> FSLGLQDFDLLRVIGRGSYAKVLLVRLKKTDRIYAMKVVKKELVNDDEDIDWVQTEKHVFEQASNHPFLVGLHSCFQTESRLFFVIEYVNGGDLMFHMQRQRKLPEEHARFYSAEISLALNYLHERGIIYRDLKLDNVLLDSEGHIKLTDYGMCKEGLRPGDTTSTFCGTPNYIAPEILRGEDYGFSVDWWALGVLMFEMMAGRSPFDIVGSSDNPDQNTEDYLFQVILEKQIRIPRSLSVKAASVLKSFLNKDPKERLGCHPQTGFADIQGHPFFRNVDWDMMEQKQVVPPFKPNISGEFGLDNFDSQFTNEPVQLTPDDDDIVRKIDQSEFEGFEYINPLLMSAEECV

Atypical protein kinase C (aPKC) is a key apical-basal polarity determinant and Par complex component. The atypical protein kinase C (aPKC in Drosophila or PKCι/PKCζ isozymes in mammals), its binding partner Par6, and the small guanosine triphosphatase Cdc42 are three essential determinants of apical membrane identity in both Drosophila and mammals (Fletcher et al., 2012, Harris and Tepass, 2008, Hutterer et al., 2004, Izumi et al., 1998, Joberty et al., 2000, Lin et al., 2000, Wodarz et al., 2000). aPKC isoforms PKCι and PKCζ have regulatory regions distinct from those of other PKC isozymes, but share a conserved catalytic protein kinase domain. Like many protein kinases, activation of aPKC requires activation-loop phosphorylation and an αC-helix conformation compatible with Lys-Glu salt-bridge formation to bind ATP and serve to align residues within the R spine (Kornev et al., 2008).

To fully understand how Par3CR3 inhibits PKCι and disrupts its activated state, we determined the structure of an “active” conformer of PKCι for comparison. We captured an active mature PKCι conformation bound to the ATP analog 5′-(β,γ-adenylyl methylene)diphosphonate (AMPPCP) at 1.8 Å. This analog was resistant to hydrolysis compared with AMPPNP. The structure has an ordered αB-αC loop and reveals side-chain contacts between Y265PKCι of the P loop and D295PKCι of the αB-αC loop. This interaction stabilizes Y265PKCι side-chain stacking with a rotamer of W298PKCι from the αC helix. Other PKC isoform structures have a phenylalanine and cysteine, respectively, at these positions (Grodsky et al., 2006, Leonard et al., 2011, Xu et al., 2004). Structural comparisons suggest that Par3CR3 inhibitory arm not only separates P-loop contacts with αB-αC loop/αC helix but also hijacks Y265PKCι and S264PKCι side chains to directly form hydrogen bonds with CR3 main-chain atoms.>[2x]ANELTWHDVLAEEKQQPYFLNTLQTVASERQSGVTIYPPQKDVFNAFRFTELGDVKVVILGQDPYHGPGQAHGLAFSVRPGIAIPP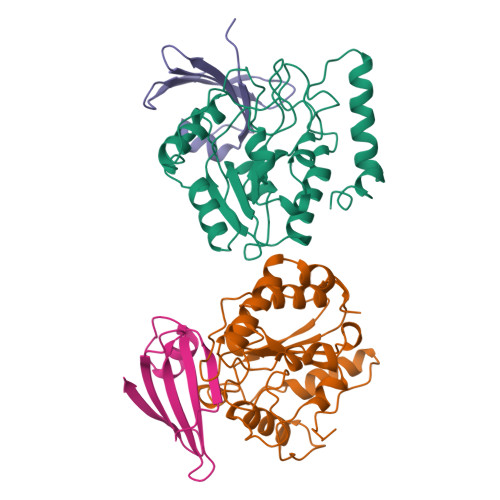SLLNMYKELENTIPGFTRPNHGYLESWARQGVLLLNTVLTVRAGQAHSHASLGWETFTDKVISLINQHREGVVFLLWGSHAQKKGAIIDKQRHHVLKAPHPSPLSAHRGFFGCNHFVLANQWLEQRGETPIDWMPVLPAESE;>MTNLSDIIEKETGKQLVIQESILMLPEEVEEVIGNKPESDILVHTAYDESTDENVMLLTSDAPEYKPWALVIQDSNGENKIKML[2x]> MHHHHHHKNIINTSILNLRYESNHLIDLSRYASEINIGSKVNFDPIDKNQIQLFNLESSKIEIILKNAIVYNSMYENFSTSFWIKIPKYFSKINLNNEYTIINCIENNSGWKVSLNYGEIIWTLQDNKQNIQRVVFKYSQMVAISDYINRWIFITITNNRLNNSKIYINGRLIDQKPISNLGNIHASNNIMFKLDGCRDPQRYIWIKYFNLFDKELNEKEIKDLYDNQSNSGILKDFWGNYLQYDKPYYMLNLYDPNKYVDVNNVGIRGYMYLKGPRGSIVTTNIYLNSSLYMGTKFIIKKYASGNKDNIVRNNDRVYINVVVKNKEYRLATNASQAGVEKILSVLEIPDVGNLSQVVVMKSKNDQGIRNKCKMNLQDNNGNDIGFIGFHQFNNIDKLVASNWYNRQIERSSRTFGCSWEFIPVDDGWGESPL

Clostridium botulinum neurotoxins (BoNTs) cause flaccid paralysis through inhibition of acetylcholine release from motor neurons; however, at tiny doses, this property is exploited for use as a therapeutic. Each member of the BoNT family of proteins consists of three distinct domains: a binding domain that targets neuronal cell membranes (HC), a translocation domain (HN) and a catalytic domain (LC).

Here, we present high‐resolution crystal structures of the binding domains of BoNT subtypes/A5 (HC/A5) and/A6 (HC/A6). These structures show that the core fold identified in other subtypes is maintained, but with subtle differences at the expected receptor‐binding sites.> DCPSGWSSYEGHCYKPFKLYKTWDDAERFCTEQAKGGHLVSIESAGEADFVAQLVTENIQNTKSYVWIGLRVQGKEKQCSSEWSDGSSVSYENWIEAESKTCLGLEKETGFRKWVNIYCGQQNPFVCE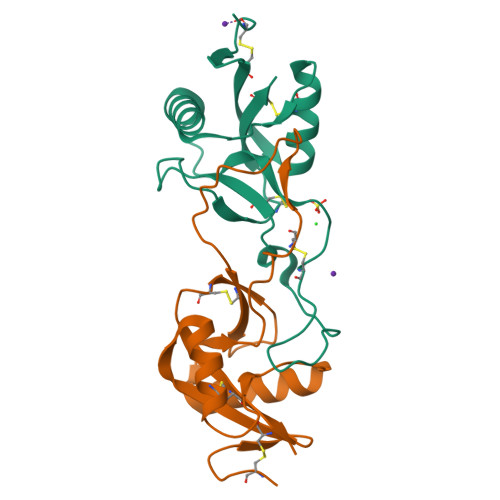A;> DCPSDWSSYEGHCYKPFSEPKNWADAENFCTQQHAGGHLVSFQSSEEADFVVKLAFQTFGHSIFWMGLSNVWNQCNWQWSNAAMLRYKAWAEESYCVYFKSTNNKWRSRACRMMAQFVCEFQA> 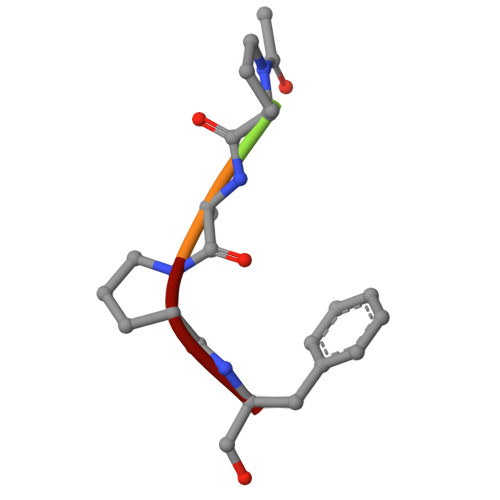XPAPF>[8x]GATITHQEKLLTVDTTAHPFLKALGGHEGTDIFPLFMDPYNGLMVMRASFAPGLTLPLHFHTGTVHMYTISGCWYYTEYPGQKQTAGCYLYEPGGSIHQFNT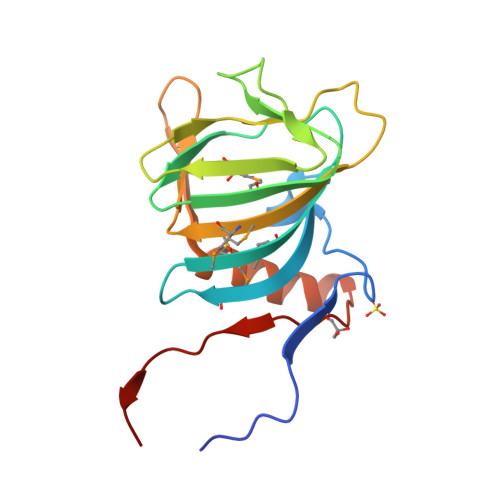PRDNEGQTEVIFMLSGCNVNFTQDGTYLGLSDAGVIKNWVDRAIREQDNGLRYIAAAVPTYAA>MADKLFINALKKKFEESPEEKKTTFYTLGGWKQSERKTEFVNAGKEVAAKRGIPQYNPDIGTPLGQRVLMPYQVSTTDTYVEGDDLHFVNNAAMQQMWDDIRRTVIVGLNHAHAVIEKRLGKEVTPETITHYLETVNHAMPGAAVVQEHMVETHPALVADSYVKVFTGNDEIADEIDPAFVIDINKQFPEDQAETLKAEVGDGIWQVVRIPTIVSRTCDGATTSRWSAMQIGMSMISAYKQAAGEAATGDFAYAAKHAEVIHMGTYLPVRRARGENEPGGVPFGYLADICQSSRVNYEDPVRVSLDVVATGAMLYDQIWLGSYMSGGVGFTQYATAAYTDNILDDFTYFGKEYVEDKYGLCEAPNNMDTVLDVATEVTFYGLEQYEEYPALLEDQFGGSQRAAVVAAAAGCSTAFATGNAQTGLSGWYLSMYLHKEQHSRLGFYGYDLQDQCGASNVFSIRGDEGLPLELRGPNYPNYAMNVGHQGEYAGISQAPHAARGDAFVFNPLVKIAFADDNLVFDFTN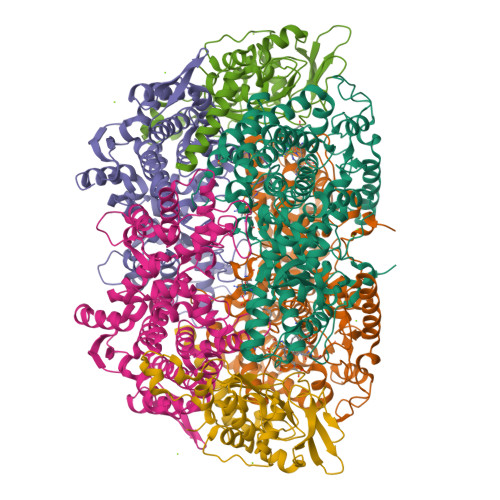VRGEFAKGALREFEPAGERALITPAK[2x];>[2x]MAKFEDKVDLYDDRGNLVEEQVPLEALSPLRNPAIKSIVQGIKRTVAVNLEGIENALKTAKVGGPACKIMGRELDLDIVGNAESIAAAAKEMIQVTEDDDTNVELLGGGKRALVQVPSARFDVAAEYSAAPLVTATAFVQAIINEFDVSMYDANMVKAAVLGRYPQSVEYMGANIATMLDIPQKLEGPGYALRNIMVNHVVAATLKNTLQAAALSTILEQTAMFEMGDAVGAFERMHLLGLAYQGMNADNLVFDLVKANGKEGTVGSVIADLVERALEDGVIKVEKELTDYKVYGTDDLAMWNAYAAAGLMAATMVNQGAARAAQGVSSTLLYYNDLIEFETGLPSVDFGKVEGTAVGFSFFSHSIYGGGGPGIFNGNHIVTRHSKGFAIPCVAAAMALDAGTQMFSPEATSGLIKEVFSQVDEFREPLKYVVEAAAEIKNEI;>[2x]MAQYYPGTTKVAQNRRNFCNPEYELEKLREISDEDVVKILGHRAPGEEYPSVHPPLEEMDEPEDAIREMVEPIDGAKAGDRVRYIQFTDSMYFAPAQPYVRSRAYLCRYRGADAGTLSGRQIIETRERDLEKISKELLETEFFDPARSGVRGKSVHGHSLRLDEDGMMFDMLRRQIYNKDTGRVEMVKNQIGDELDEPVDLGEPLDEETLMEKTTIYRVDGEAYRDDVEAVEIMQRIHVLRSQGGFNLE NRTIs mimic natural deoxynucleosides or deoxynucleotides and target the reverse transcriptase (RT) enzyme. RT incorporates active metabolites of NRTIs into the growing DNA chain which act as chain terminators due to their lack of 3ʹ-OH. M184 is part of the conserved active site YMDD motif found in several viral polymerases, including HIV-1 RT and HBV polymerase. Herein, using the same DNA construct, we report the pre-steady-state kinetic analysis with WT RT and M184V to determine the incorporation efficiency of both (+)- and (−)-enantiomers of FTC-TP and 3TC-TP compared to dCTP in addition to crystal structures of WT RT in complex with dsDNA (RT–DNA) bound to either, (−)-FTC-TP, (−)-3TC-TP, (+)-FTC-TP, or dCTP.

Overall, the positions of the cytidine and oxathiolane are similar as in the RT–DNA•(−)-FTC-TP structure. There is only one conformation of the triphosphates observed which matches the non-productive conformation observed in RT–DNA•(−)-FTC-TP and RT–DNA•(−)-3TC-TP. As with the RT–DNA•(−)-FTC-TP, there is a Mg2+ ion with an octahedral ligand coordination sphere observed; however the Mg2+ interacts with the α- and γ-phosphates and not the β-phosphate. Because the β-phosphate is shifted and not interacting with the Mg2+, a water molecule was observed completing the coordination sphere. Examining the van der Waals radius of V184, it is clear that there is a direct interaction with the branched side chain and the sulfur in the oxathiolane ring of (−)-FTC-TP. For the RT–DNA•(−)-FTC-TP complex, the closest distance of the oxathiolane ring to M184 was 4.1 Å, compared to 3.4 Å for the valine side chain. Structure alignment through residues 107–112 and 151–215 in the p66 subunit between the WT and M184V structures with (−)-FTC-TP shows that the oxathiolane sulfur is shifted away from residue V184 by 0.3 Å compared to M184. A concerted movement is observed in (−)-FTC-TP that results in the C5´ carbon, which is the pivot point of the different triphosphate orientations, further shifting by 0.6 Å. Although the calculated maximum likelihood coordinate error reported in Phenix refinement is 0.33 Å for the WT and M184V (−)-FTC-TP structures, this shift is propagated to cause other atoms of (−)-FTC-TP to move more than 0.33 Å from the WT structure. The combination of a steric shift and altered triphosphate orientation likely results in reduced binding affinity of (−)-FTC-TP (280-fold higher Kd in Table 1) with M184V than with WT RT.

> MGSSHHHHHHSSPISPIETVPVKLKPGMDGPKVKQWPLTEEKIKALVEICTEMEKEGKISKIGPENPYNTPVFAIKKKDSTKWRKLVDFRELNKRTQDFWEVQLGIPHPAGLKKKKSVTVLDVGDAYFSVPLDEDFRKYTAFTIPSINNETPGIRYQYNVLPQGWKGSPAIFQSSMTKILEPFRKQNPDIVIYQYVDDLYVGSDLEIGQHRTKIEELRQHLLRWGLTTPDKKHQKEPPFLWMGYELHPDKWTVQPIVLPEKDSWTVNDICKLVGKLNWASQIYPGIKVRQLSKLLRGTKALTEVIPLTEEAELELAENREILKEPVHGVYYDPSKDLIAEIQKQGQGQWTYQIYQEPFKNLKTGKYARMRGAHTNDVKQLTEAVQKITTESIVIWGKTPKFKLPIQKETWETWWTEYWQATWIPEWEFVNTPPLVKLWYQLEKEPIVGAETFYVDGAANRETKLGKAGYVTNRGRQKVVTLTDTTNQKTELQAIYLALQDSGLEVNIVTDSQYALGIIQAQPDQSESELVNQIIEQLIKKEKVYLAWVPAHKGIGGNEQVDKLVSAGIRKVL;> PISPIETVPVKLKPGMDGPKVKQWPLTEEKIKALVEICTEMEKEGKISKIGPENPYNTPVFAIKKKDSTKWRKLVDFRELNKRTQDFWEVQLGIPHPAGLKKKKSVTVLDVGDAYFSVPLDEDFRKYTAFTIPSINNETPGIRYQYNVLPQGWKGSPAIFQSSMTKILEPFRKQNPDIVIYQYVDDLYVGSDLEIGQHRTKIEELRQHLLRWGLTTPDKKHQKEPPFLWMGYELHPDKWTVQPIVLPEKDSWTVNDIQKLVGKLNWASQIYPGIKVRQLSKLLRGTKALTEVIPLTEEAELELAENREILKEPVHGVYYDPSKDLIAEIQKQGQGQWTYQIYQEPFKNLKTGKYARMRGAHTNDVKQLTEAVQKITTESIVIWGKTPKFKLPIQKETWETWWTEYWQATWIPEWEFVNTPPLVKLWYQLEKEPIVGAETF> MVARVQTAEEIRDEGNAAVKDQDYIKADELYTEALQLTTDEDKALRPVLYRNRAMARLKRDDFEGAQSDCTKALEFDGADVKALFRRSLAREQLGNVGPAFQDAKEALRLSPNDKGIVEVLQRLVKANNDKIKQTTSLANKVTDMEKLAFRGEAKDTEQKMTALNNLLVLCRESESGATGVWNQGALVPFVLNLINDASENE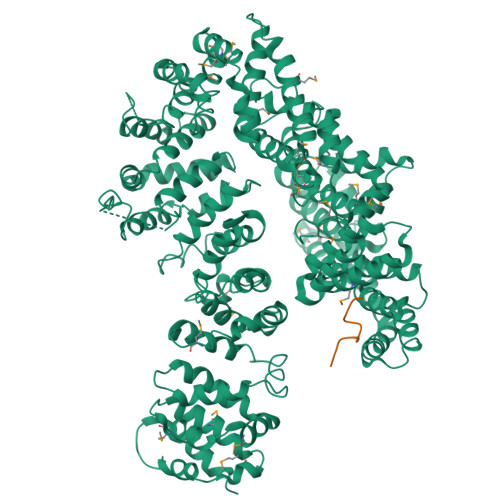EVTVTAIRILDETIKNSVRCMKFLAMHDPDGPKSVRFVCRLMCKKSTKDFVDATGILVQRVFNAMAKMDRQKEMKPDPEVAEANKIWIIRVLLELQEMLQDPKVGAVQRETCIDLFLKNLMHMDGGIPRGWSWKFVEERGLLALLDVASQIPELCEYPVSAETRQHVAICLQRLEEDMVFDTKRTIFKEKVDMFFNALISRCTNDDEGHKYRIKLSCFLITMLQGPVDIGINLITNDQLTPIMLEMAASQDHLMQGIAAELIVATVSKHERAINMLKVGIPVLRALYDSEDPTVKVRALVGLCKIGAAGGDDISKATMKEEAVISLAKTCKKFLLETEKYSVDIRRYACEGLSYLSLDADVKEWIVDDSLLLKALVLLAKKAGALCVYTLATIYANLSNAFEKPKVDEEMVKLAQFAKHHVPETHPKDTEEYVEKRVRALVEEGAVPACVAVSKTESKNALELIARSLLAFAEYEDLRGRIIAEGGTVLCLRLTKEASGEGKIKAGHAIAKLGAKADPMISFPGQRAYEVVKPLCDLLHPDVEGKANYDSLLTLTNLASVSDSIRGRILKEKAIPKIEEFWFMTDHEHLRAAAAELLLNLLFFEKFYEETVAPGTDRLKLWVLYSAEVEEERLSRASAAGFAILTEDENACARIMDEIKSWPEVFKDIAMHEDAETQRRGLMGIANIMHSSNKLCSEIVSSEVFRVLVAVTKLGTINQERAGSTEQAKRGLEAAEKFGLIKATDREIYERENQMSTIQE;> AGGPTIEEVD>[4x]MKKLFLVFWWHMHQPLYREPYTGEYLLPWTFFHAVKDYYDMPAYLKDFEIKLNFNLTPVLIDQIQEYAQGKAKDVFLEAIRKDPDDLEKEEVEKLIEFTKLNYEKPIYRFERIRELMNKEKLNREELLDLQTLNLLAWCGRTLRKDLKDLLN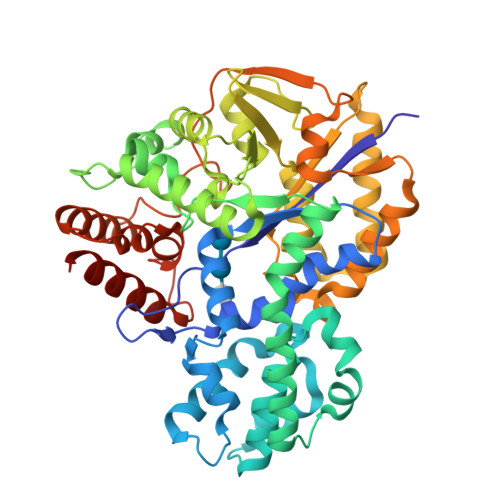KGRNYTQEEKEYVLNKYFEIIKKTLSIYREIKEEGKGSVSTSPYYHPLIPILLNPNCVYETTPNVKIPDFAVSFREDASKHVELAKEKYFEIFGEHPVYMWPPEASVSNEALELYYEKGINMLATDEVILKNSVERASPYLRYYFRELISVFFRDKTLSDLIGFSYHAWNAEDAVRDFIGRLKKIHESVDFQPVVFVVLDGENCWEYYEENGIPFLEKLYSTLEKEEWIETLTLEEAMRKEDVKTEVIESVKAGTWFDGNFLKWIGNKEKNEYWKILIEAKKKAKNDYILVAEGSDWFWWQGEEKAPFVEVFDKLFRSFVRRAQELEHHHHH>[3x]MHHHHHHSGAFEFKLPDIGEGIHEGEIVKWFVKPGDEVNEDDVLCEVQNDKAVVEIPSPVKGKVLEILVPEGTVATVGQTLITLDAPGYENMTASSSGSENLYFQGSHMTATDSSILNQYLVGKEPFYQPQHDEVALFEAAYRKRLPVMVKGPTGCGKSRFVEFMAWRLGKPLVTVACNEDMTAADLVGRWLLDKDGTRWQDGPLTVAARYGAI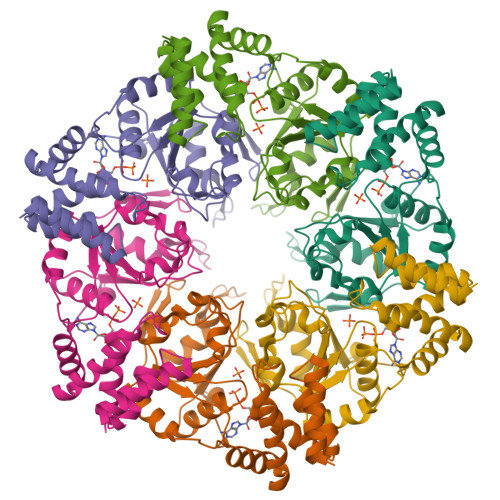CYLDEIVEARQDTTVVIHPLTDHRRTLPLDKKGELIRAHPDFQLVISYNPGYQSLMKDLKQSTKQRFTGFEFDYPNAELEAGILVQETGVAPSIAAQLVTVAATARRLKGHGLDEGISTRLLVYAAMLMDDGVAPRAACRMALVQPITDDADIRATLEHAIDMTFA The most widespread of these mechanisms employs a “controller” (C) protein encoded by a gene downstream of its own promoter, and usually co-transcribed with the endonuclease (R) gene as a single transcriptional unit. The C-protein binds at various sites within the C/R promoter to regulate transcription of its own gene and the associated endonuclease gene. Unusually, in the RM system Esp1396I, the C-protein also represses the MTase (M) gene by binding to the promoter at the transcriptional start site, denoted OM where the C/R genes and the M gene are transcribed convergently from different promoters. Flexibility in this loop is very important for DNA sequence recognition, as it has been observed in the nucleoprotein structures to adopt different conformations depending on which operator site the protein is bound to.

Of the mutant proteins, Y37F showed the strongest binding to the OM site, followed by S52A and Y37A. SPR analysis showed that Y37F formed much more stable complexes with the OM operator site than Y37A, with KDs of 1.8 and 5.5 nM respectively, but both were less stable than the wild type (KD = 0.51 nM). This indicated that the role of the tyrosine was more than just the formation of a hydrogen bond with the DNA backbone, but also involved the phenyl ring common to both tyrosine and phenylalanine. For the hydroxyl group only, the ΔΔG between the wild type and Y37F mutant was found to be −3.1 kJ mol−1 (−1.55 kJ mol−1 per hydrogen bond). The free protein structures of the wild type, Y37F and Y37A mutants showed no major structural differences either in the local binding regions in terms of helix or side chain positions, or in the overall fold. The Y37F crystal structure has six monomers (three biological dimers) in the asymmetric unit. Five of the monomers in the asymmetric unit are observed to be in loop conformation I but the sixth more closely resembles that of conformation II, which is almost identical to that in the DNA-protein complex with the 19OM operator site. Despite Y37F and T36A only crystallising in the presence of SO4, this anion was not visible in either electron density map. As with the high-resolution wild type structure, the C-terminal tail is also involved in several crystal contacts with multiple monomers in the T36A, Y37F and trigonal R46A structures.

>[6x]GSHMESFLLSKVSFVIKKIRLEKGMTQEDLAYKSNLDRTFISGIERNSRNLTIKSLELIMKGLEVSDVVFFEMLIKEILKHD> SPFSVKVGLAQMLRGGVIMDVVNAEQARIAEEAGACAVMALERVPADIRAQGGVARMSDPQMIKEIKQAVTIPVMAKARIGHFVEAQILEAIGIDYIDESEVLTLADEDHHINKHNFRIPFVCGCRNLGEALRRIREGAAMIRTKGEAGTGNIIEAVRHVRSVNGDIRVLRNMDDDEVFTFAKKLAAPYDLVMQTKQLGRLPVVQFAAGGVATPADAALMMQLGCDG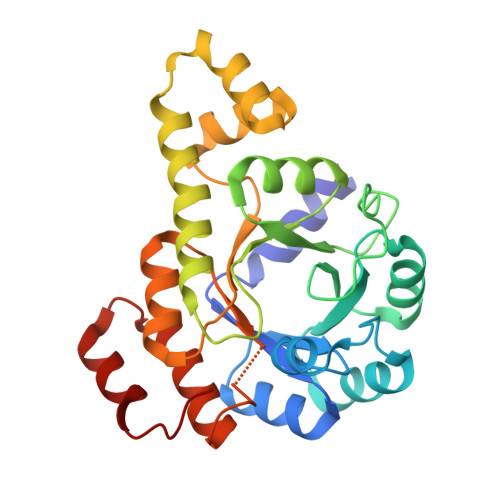VFVGSGIFKSGDPARRARAIVQAVTHYSDPEMLVEVSCGLGEAM>AECSVDIQGNDQMQFNTNAITVDKSCKQFTVNLSHPGNLPKNVMGHNWVLSTAADMQGVVTDGMASGLDKDYLKPDDSRVIAHTKLIGSGEKDSVTFDVSKLKEGEQYMFFCTPPGHSALMK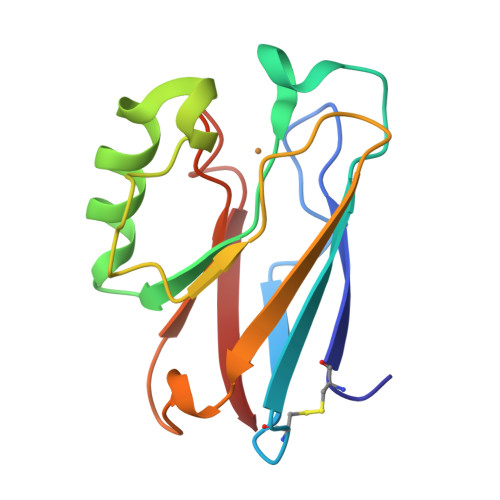GTLTLK[2x]(2R)-5-FLUORO-2-(2-THIENYL)-1,2-DIHYDROQUINAZOLIN-4-AMINE | C12 H10 F N3 S | 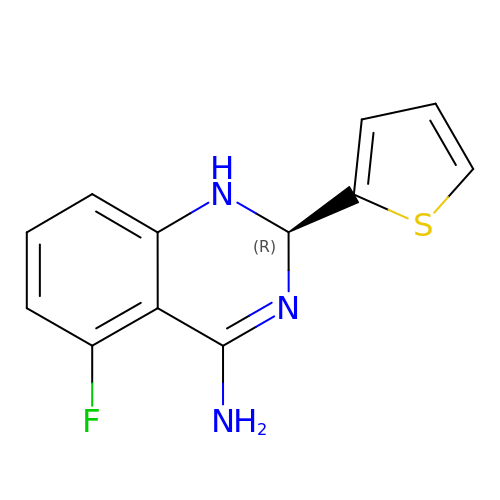OGKZGPSVQKXXOY-GFCCVEGCSA-N Growth factor receptor-bound protein 7 (Grb7) is an adaptor protein that is important in breast cancer cell migration and proliferation. Grb7 mediates interactions between autophosphorylated receptor tyrosine kinase (RTK) and downstream signalling molecules. Grb7 primarily interacts with its upstream signalling partners through its Src homology 2 (SH2) domain, leading to Grb7 tyrosine phosphorylation and signal transduction. It has therefore been hypothesised that inhibiting the Grb7-SH2 domain would inhibit breast cancer cell migration as well as other Grb7-SH2-related signal transduction pathways.

Therefore, the Phe9 and Pro10 that had previously been removed to rigidify the scaffold were re-added to the peptide. Therefore, to assess the mode of binding of G7-B8 to Grb7-SH2, the structure of the Grb7-SH2/G7-B8 complex was determined to a 2.55 Å resolution using X-ray crystallography. Interestingly, the complex crystallised with four protein molecules in the asymmetric unit, of which only two Grb7-SH2 domains were formed in complex with the peptide. The other two protein molecules remained as apo-proteins, as similarly observed for G7-18NATE bound to the Grb7-SH2 domain. The mode of G7-B8’s interaction with the Grb7-SH2 domain was strikingly similar to that previously observed for G7-18NATE, as would be expected for this peptide that differs by only two amino acids. Asn7 formed hydrogen bond interactions with the Grb7-SH2 domain Leu481, which is understood to underlie the Grb7-SH2 domain specificity for the “YXN” motif. Only amino acids 1 and 8 differed in their positioning relative to G7-18NATE due to their substitution with Lys and Glu residues in G7-B8 for the formation of the lactam ring. This linkage can be seen clearly within the G7-B8 electron density and reveals that it serves well to support the adopted conformation for the interaction with Grb7-SH2, underlying its enhanced binding affinity. Notably, G7-B8, which is most similar in sequence to G7-18NATE, was found to possess the highest affinity of the three, with a KD of 0.86 µM. The G7-B8 peptide, however, bound in the expected orientation, making the same contacts with the surface of the Grb7-SH2 domain as first observed for G7-18NATE. It can thus be concluded that the lactam linkage, unlike the more hydrophobic olefin staple, did not outcompete Phe9-Pro10 to form surface contacts with the Grb7-SH2 domain.

>[4x]GSPASGTSLSAAIHRTQLWFHGRISREESQRLIGQQGLVDGLFLVRESQRNPQGFVLSLCHLQKVKHYLILPSEEEGRLYFSMDDGQTRFTDLLQLVEFHQLNRGILPCLLRHCCTRVAL;>[2x]KFEGYDNEFPX>[3x]MAQLALQM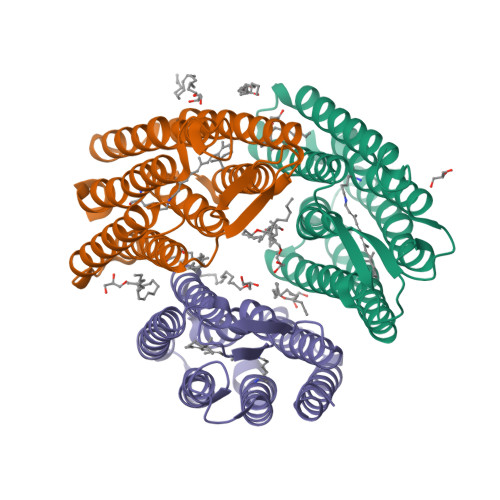SSLGVEGEGIWLALGTIGMLLGMLYFIADGLDVQDPRQKEFYVITILIPAIAAASYLSMFFGFGLTEVSLANGRVVDVYWARYADWLFTTPLLLLDIGLLAGASQRDIGALVGIDAFMIVTGLVATLTKVVVARYAFWTISTISMVFLLYYLVAVFGEAVSDADEDTRSTFNALRNIILVTWAIYPVAWLVGTEGLALTGLYGETLLFMVLDLVAKVGFGFILLRSRAIMGGGSEPTPSAQETAADLEHHHHHH> MSTETLEIYRKALNFNVIARYDPKIKQLLFHTPHATVYKWGDDNWNKLEYQGVLAIYLRDVGDKEAILPEVSSYDDTITGQQSEANTPHVLTGHDIYNYGLIIMNRINPDNFSLAIAPNSVLN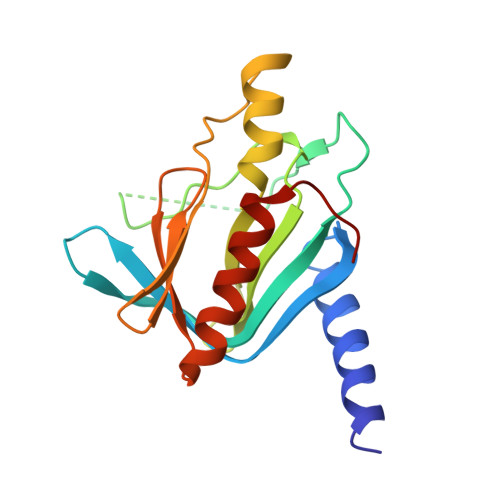KRKLFAPNREEELEPMKVEVRDDLVMIKTLKKEVYGIWVHTPEDRQNIYELIKYLLENEPTDSFT>[2x]HLVCPMSKSPYVDPHKSGHEIWEEFSMSFTPAVKEVVEFAKRIPGFRDLSQHDQVNLLKAGTFEVLMVRFASLFDAKERTVTFLSGKKYSVDDLHSMGAGDLLNSMFEFSEKLNALQLSDEEMSLFTAVVLVSADRSGIENVNSVEALQETLIRALRTLIMKNHPNEASIFTKLLLKLPDLRSLNNMHSEELLAFKVHP;>[2x]RTHRLITLADHICQIITQDFARN

The REV-ERBs, REV-ERBα (NR1D1) and REV-ERBβ (NR1D2), are closely related NRs with critical roles in mammalian physiology, including maintenance of the circadian rhythm, metabolic processes, and immune function. The REV-ERBs are unique among NRs because their ligand-binding domains (LBDs) lack the C-terminal activation function–2 (AF-2) helix 12 important for binding transcriptional coactivator proteins, suggesting that the REV-ERBs should interact exclusively with transcriptional corepressor proteins and solely repress transcription. The iron-centered porphyrin heme has been identified as the endogenous REV-ERB ligand. REV-ERB LBD interacts with NCoR via two ID motifs present within the RID.

Ligand-free (apo) REV-ERBβ LBD exhibited high affinity for ID1 peptide and low affinity for ID2 peptide. Heme decreased LBD affinity for the ID1 peptide but increased LBD affinity for ID2 peptide, effectively equalizing the ID1 and ID2 peptide affinities. To determine the structural basis of this interaction, we solved crystal structures of REV-ERBβ LBD cobound to heme and NCoR ID1 peptide (2.6-Å resolution) or ID2 peptide (2.0-Å resolution) (respectively). In both structures, REV-ERBβ LBD crystallized with two molecules in the asymmetric unit with an NCoR ID peptide and heme molecule cobound to each LBD. The overall root mean square deviation (RMSD) of the complex in the asymmetric unit including LBD, heme, and NCoR ID peptide was 1.1 and 1.3 Å for the ID1- and ID2-bound structures, respectively, suggesting minimal conformational heterogeneity. The ID peptides bound to the AF-2 surface formed electrostatic interactions with the conserved charge clamp residue K421 on helix 3, confirming that the heme-dependent REV-ERBβ corepressor interaction is similar to other NRs. The overall heme-bound LBD conformations were largely unchanged by peptide binding, with average LBD RMSDs of 1.0 and 1.3 Å for the ID1- and ID2-bound structures, respectively, relative to the published heme-bound LBD structure. In the crystal structure of apo REV-ERBα LBD bound to NCoR ID1 peptide, an antiparallel β sheet is formed between the N terminus of the ID1 peptide and a β strand extension off helix 11 (10). Although the antiparallel β sheet was lost, the AF-2 interaction with the α-helical region of the ID1 and ID2 peptides containing the I/LxxI/LI/LxxxI/L/F corepressor NR (CoRNR) box motif critical for corepressor binding was preserved. Heme binding inhibits formation of the antiparallel β sheet, which likely contributes to higher-affinity ID1 binding to the apo LBD, resulting in lower-affinity ID1 binding to heme-bound LBD.> GGGAGUCGGGUCUGUGGUUG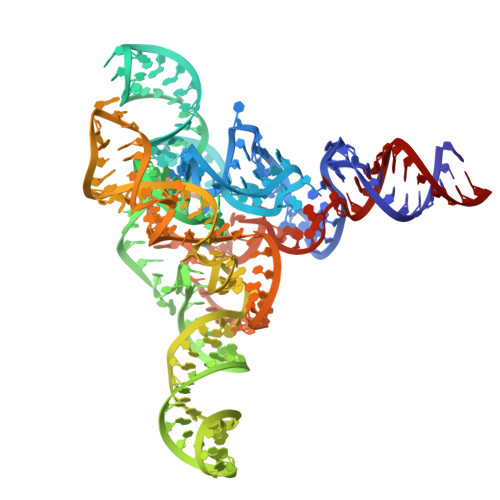AAAGUCGAUGCCAGUCGCAGGCGAAACGAUCCACAUAAGCGGGGCAAAGUUCCCGUGAGCAUGGUGCGGCUUAGAUGUAAGUCCUGUCGUGCGGCAUUCCGAAUCGAAUGCGGUGCGAGAGUGGCAGUAGUGGGCGGCGUAAAGCUCAGUAGCGAACCCACCGACAGGCGAGUGUGGGGGCAAAAACCAGGUCAGCCGACUCCA> MHHHHHHENLYFQSTKPFFDAARVIAGGKLTQAQVDDLNKVVEKLAPGGKTTSDDGIDLITSFEGTRFNAYDDGVGVWTIGTGTTVYPNGVKVKKGDTCTAEQAKTYFKHDLAKFEKTVNESVTAPLTQNQFDALVSLTYNIGSGAFNNSTLLKKLNKG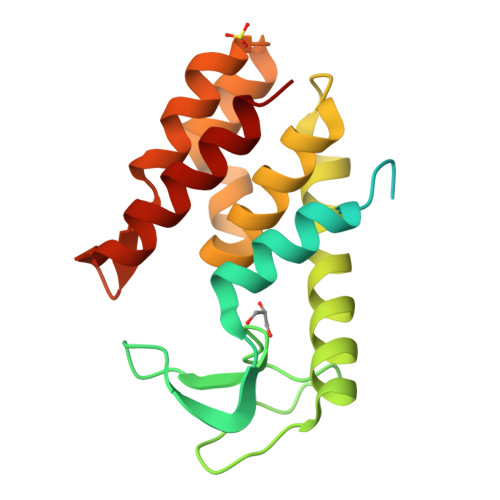DYQGAADQFLVWNKAGGKVMKGLVRRREAERALFLKK> KRYSALSNDISQGIKRQRMTVESMGWALS;> MGSMAMDTFITRNFQTTI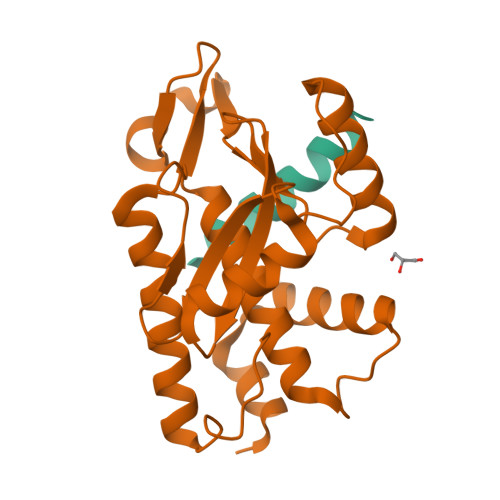IQKAKNTMAEFSEDPELQPAMLFNICVHLEVCYVISDMNFLDEEGKSYTALEGQGKEQNLRPQYEVIEGMPRTIAWMVQRSLAQEHGIETPKYLADLFDYKTKRFIEVGITKGLADDYFWKKKEKLGNSMELMIFSYNQDYSLSNESSLDEEGKGRVLSRLTELQAELSLKNLWQVLIGEEDVE N-CYCLOHEXYL-N'-(4-IODOPHENYL)UREA | C13 H17 I N2 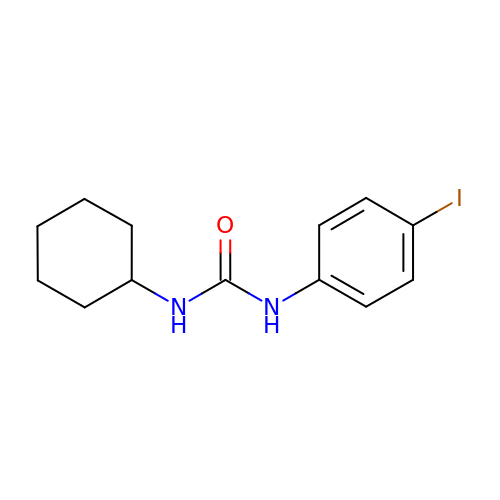O | AQTBUVAFYDVTFD-UHFFFAOYSA-N>[2x]MRNRREVSKLLSERVLLLDGAYGTEFMKYGYDDLPEELNIKAPDVVLKVHRSYIESGSDVILTNTFGATRMKLRKHGLEDKLDPIVRNAVRIARRAAGEKLVFGDIGPTGELPYPLGSTLFEEFYENFRETVEIMVEEGVDGIIFETFSDILELKAAVLAAREVSRDVFLIAHMTFDEKGRSLTGTDPANFAITFDELDIDALGINCSLGPEEILPIFQELSQYTDKFLVVEPNAGKPIVENGKTVYPLKPHDFAVHIDSYYELGVNIFGGCCGTTPEHVKLFRKVLGNRKPLQRKKKRIFAVSSPSKLVTFDHFVVIGERINPAGRKKLWAEMQKGNEEIVIKEAKTQVEKGAEVLDVNFGIESQIDVRYVEKIVQTLPYVSNVPLSLDIQNVDLTERALRAYPGRSLFNSAKVDEEELEMKINLLKKYGGTLIVLLMGKDVPKSFEERKEYFEKALKILERHDFSDRVIFDPGVLPLGAEGKPVEVLKT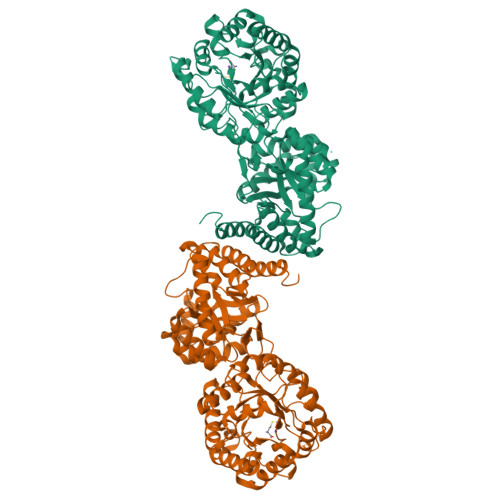IEFISSKGFNTTVGLSNLSFGLPDRSYYNTAFLVLGISKGLSSAIMNPLDETLMKTLNATLVILEKKELPRAEVK Here, we perform structural and biochemical characterization of the Legionella pneumophila effector Lpg2370, demonstrating that it is a Ser/Thr kinase. Together with two upstream genes, lpg2370 constitutes the tripartite HipBST TA. Notably, the toxin Lpg2370 (HipTLp) and the antitoxin Lpg2369 (HipSLp) correspond to the C-terminus and N-terminus of HipA from HipBA TA, respectively. Structural analysis reveals that HipSLp binding induces a loop-to-helix shift in the P-loop of HipTLp, leading to the blockage of ATP binding and inhibition of the kinase activity.

In this work, we find that Lpg2370 in fact shares sequence identity with the C-terminus of the E. coli K-12 HipA, the toxin of type II TA system HipBA, which is then confirmed by experimental validation and determining the crystal structure of autophosphorylated Lpg2370 (pLpg2370). Like other members of the protein kinase superfamily, Lpg2370 has a globular kinase fold that can be further divided into N-lobe and C-lobe. The N-lobe, which contains the P-loop, is composed of sheets β1–5 sandwiched by helices α1 and α2, whereas the C-lobe is predominantly α-helical and consists of helix bundles α3–α6 and α8–α11 and a short β-sheet β6–8. In agreement with our LC-MS/MS results, we can observe a phosphate group covalently attached to the Ser54 residue. However, unlike HipAEc and HipASo whose P-loops are disordered upon serine autophosphorylation, the electron density of the Lpg2370 P-loop is well defined in the present structure. One prominent difference is that the Lpg2370 P-loop with phosphorylated Ser54 is exposed to solvent in an orientation similar to that of unphosphorylated P-loop of HipAEc, which upon serine autophosphorylation rotates by ~180° and bends away from the N-terminal lobe by 17.3 Å. Lpg2370 and HipAEc superimpose with a relatively large root-mean-square deviation (RMSD) value of 3.846 Å over 221 Cα atoms. Conversely, the six C-terminal α-helices of Lpg2370 and HipAEc, including the catalytic residues and some ATP-binding residues, are almost perfectly aligned. A comparison of the crystal structure of pHipTLp and the structures deposited in the PDB revealed that the autophosphorylated P-loop in HipTLp adopts an orientation similar to that of the P-loop in the crystal structure of E. coli HipA S150A mutant.

> FQSNAMKHCPITYEKISDQENYSQRGLHLLSPQLKNLSPLDLSADEQRQEAIARVGKMSVQGVQKKLSAKLKIKEGCFEIVDQYGQYILKPQSDIYPELPENEAITMTLAKTIGLEVPVHGLVYSKDNSLTYFIKRFDRIGHNKKLALEDFAQLSGEDRHTKYKSSMEKVIAVIEQFCTFPKIEFVKLFKLTLFNFLVGNEDMHLKNFSLITKDRKISISPAYDLLNSTIAQKNTKEELALPLKGKKNNLTKSDFLKYFAIEKLGLNQNVIDGIVQEFHQVIPKWQELIGFSFLSQEMQEKYLELLEQRCKRLNFFD> SGIVPTLQNIVATVTL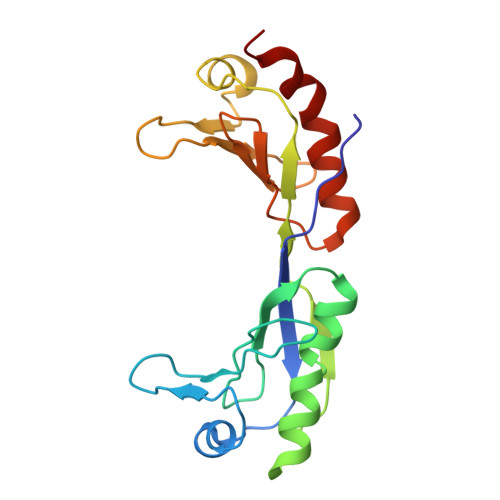GCRLDLKTVALHARNAEYNPKRFAAVIMRIREPKTTALIFASGKMVVTGAKSEDDSKLASRKYARIIQKIGFAAKFTDFKIQNIVGSCDVKFPIRLEGLAFSHGTFSSYEPELFPGLIYRMVKPKIVLLIFVSGKIVLTGAKQREEIYQAFEAIYPVLSEFRKM> 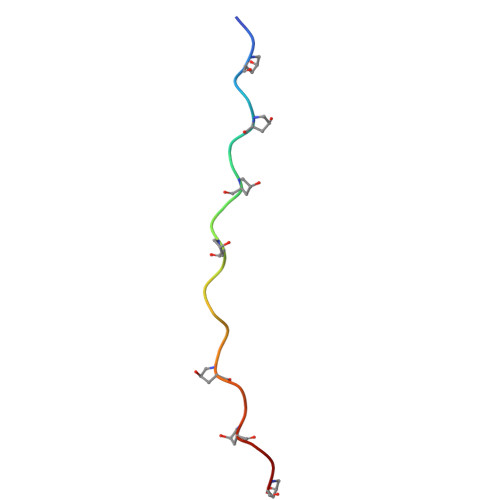GPPGPPGPPGVPGEAGPPGPPGPP> MKISVSKNDLENALRYLQAFLDKKDASSIASHIHLEVIKEKLFLKASDSDIGLKSYIFTQSSDKEGVGTINGKKFLDIISCLKDSNIILETKDDSLAIKQNKSSFKLPMFDADEFPEFPVIDPKVSIEVNAPFLVDAFKKIAPVIEQTSHKRELAGILMQFDQKHQTLSVVGTDTKRLSYTQLEKISIHSTEEDISCILPKRALLEILKLFYENFSFKSDGMLAVIENEMHTFFTKLIDGNYPDYQKILPKEYISSFTLGKEEFKESIKLCSSLSSTIKLTLEKNNALFESLDSEHSETAKTSVEIEKGLDIEKAFHLGVNAKFFLEALNALGTTQFVLRCNEPSSPFLIQESLDEKQSHLNAKISTLMMPITLLEHHHHHH

The sliding clamp is a ring-shaped protein complex that encircles DNA with the help of clamp loader in an ATP-dependent manner, and slides along the DNA. In prokaryotes, however, β-clamp is a homodimer, with each monomer consisting of three globular domains, and in this way β-clamp displays a six-domain ring. Although β-clamp is part of the DNA polymerase III holoenzyme, it is not attached to polymerase III permanently like the other subunits. β-clamp is loaded on the DNA, by clamp loader, a subunit of DNA Pol III. In both prokaryotes and eukaryotes, a key feature of this clamp-binding motif is the presence of hydrophobic amino acid residues that bind to the hydrophobic pocket in the C-terminal region of the clamp.

In the space group C2, one monomer was observed in each asymmetric unit, which interacts with another monomer from asymmetric unit to form a dimer. However there is no significant difference observed between these two structures from different space groups, the structural alignment of both yielded an RMSD of 0.15 Å. While Hpβ-clamp was found to exist as both a monomer and dimer in the crystal, the dimer was the dominant component in solution according to a gel filtration experiment. The dimeric ring shaped structure is a biological functional unit that binds to DNA and slides along the DNA. As in other clamps, twelve alpha helices were observed to form the inner surface of the Hpβ-clamp ring, with positively charged residues suitable for binding DNA. The β-sheets along with loops were found to form the outer surface of the ring. The N-terminal region of Hpβ-clamp was found to have more electropositive residues and the C-terminal region more electronegative residues at the dimeric interface. Although superposition revealed the overall structure of Hpβ-clamp to be similar to the β-clamp structures in other organisms, but some important differences are there at the regions involved in DNA binding. In domain II, the loop containing residues 210–214 was observed to be shorter in Hpβ-clamp than in E. coli and the other homologs. Moreover, in E. coli and the other homologs, the B-factor for this region was found to be quite high, compared to that for the other regions in the protein, in contrast to the case in H. pylori. These results indicate that this loop in other organism may interact with DNA, however this shortened loop in H. pylori may not be involved in DNA interactions because of the absence of certain residues.>MYSTAVLLNKISPTRDGQTMTLADLQYLSFSELRKIFDDQLSWGEARHLYHETIEQKKNNRLLEARIFTRANPQLSGAIRLGIERDSVSRSYDEMFGARSSSFVKPGSVASMFSPAGYLTELYREAKDLHFSSSAYHLDNRRPDLADLTLSQSNMDTEISTLTLSNELLLEHITRKTGGDSDALMESLSTYRQAIDTPYHQPYETIRQVIMTHDSTLSALSRNPEVMGQAEGASLLAILANISPELYNILTEEITEKNADALFAQNFSENITPENFASQSWIAKYYGLELSEVQKYLGMLQNGYSDSTSAYVDNISTGLVVNNESKLEAYKITRVKTDDYDKNINYFDLMYEGNNQFFIRANFKVSREFGATLRKNAGPSGIVGSLSGPLIANTNFKSNYLSNISDSEYKNGVKIYAYRYTSSTSATNQGGGIFTFESYPLTIFALKLNKAIRLCLTSGLSPNELQTIVRSDNAQGIINDSVLTKVFYTLFYSHRYALSFDDAQVLNGSVINQYADDDSVSHFNRLFNTPPLKGKIFEADGNTVSIDPDEEQSTFARSALMRGLGVNSGELYQLGKLAGVLDAQNTITLSVFVISSLYRLTLLARVHQLTVNELCMLYGLSPFNGKTTASLSSGELPRLVIWLYQVTQWLTEAEITTEAIWLLCTPEFSGNISPEISNLLNNLRPSISEDMAQSHNRELQAEILAPFIAATLHLASPDMARYILLWTDNLRPGGLDIAGFMTLVLKESLNANETTQLVQFCHVMAQLSLSVQTLRLSEAELSVLVISGFAVLGAKNQPAGQHNIDTLFSLYRFHQWINGLGNPGSDTLDMLRQQTLTADRLASVMGLDISMVTQAMVSAGVNQLQCWQDINTVLQWIDVASALHTMPSVIRTLVNIRYVTALNKAESNLPSWDEWQTLAENMEAGLSTQQAQTLADYTAERLSSVLCNWFLANIQPEGVSLHSRDDLYSYFLIDNQVSSAIKTTRLAEAIAGIQLYINRALNRIEPNARADVSTRQFFTDWTVNNRYSTWGGVSRLVYYPENYIDPTQRIGQTRMMDELLENISQSKLSRDTVEDAFKTYLTRFETVADLKVVSAYHDNVNSNTGLTWFVGQTRENLPEYYWRNVDISRMQAGELAANAWKEWTKIDTAVNPYKDAIRPVIFRERLHLIWVEKEEVAKNGTDPVETYDRFTLKLAFLRHDGSWSAPWSYDITTQVEAVTDKKPDTERLALAASGFQGEDTLLVFVYKTGKSYSDFGGSNKNVAGMTIYGDGSFKKMENTALSRYSQLKNTFDIIHTQGNDLVRKASYRFAQDFEVPASLNMGSAIGDDSLTVMENGNIPQITSKYSSDNLAITLHNAAFTVRYDGSGNVIRNKQISAMKLTGVDGKSQYGNAFIIANTVKHYGGYSDLGGPITVYNKTKNYIASVQGHLMNADYTRRLILTPVENNYYARLFEFPFSPNTILNTVFTVGSNKTSDFKKCSYAVDGNNSQGFQIFSSYQSSGWLDIDTGINNTDIKITVMAGSKTHTFTASDHIASLPANSFDAMPYTFKPLEIDASSLAFTNNIAPLDIVFETKAKDGRVLGKIKQTLSVKRVNYNPEDILFLRETHSGAQYMQLGVYRIRLNTLLASQLVSRANTGIDTILTMETQRLPEPPLGEGFFANFVLPKYDPAEHGDERWFKIHIGNVGGNTGRQPYYSGMLSDTSETSMTLFVPYAEGYYMHEGVRLGVGYQKITYDNTWESAFFYFDETKQQFVLINDADHDSGMTQQGIVKNIKKYKGFLNVSIATGYSAPMDFNSASALYYWELFYYTPMMCFQRLLQEKQFDEATQWINYVYNPAGYIVNGEIAPWIWNCRPLEETTSWNANPLDAIDPDAVAQNDPMHYKIATFMRLLDQLILRGDMAYRELTRDALNEAKMWYVRTLELLGDEPEDYGSQQWAAPSLSGAASQTVQAAYQQDLTMLGRGGVSKNLRTANSLVGLFLPEYNPALTDYWQTLRLRLFNLRHNLSIDGQPLSLAIYAEPTDPKALLTSMVQASQGGSAVLPGTLSLYRFPVMLERTRNLVAQLTQFGTSLLSMAEHDDADELTTLLLQQGMELATQSIRI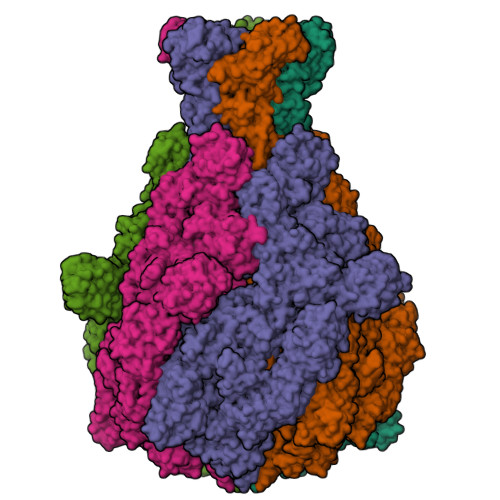QQRTVDEVDADIAVLAESRRSAQNRLEKYQQLYDEDINHGEQRAMSLLDAAAGQSLAGQVLSIAEGVADLVPNVFGLACGGSRWGAALRASASVMSLSATASQYSADKISRSEAYRRRRQEWEIQRDNADGEVKQMDAQLESLKIRREAAQMQVEYQETQQAHTQAQLELLQRKFTNKALYSWMRGKLSAIYYQFFDLTQSFCLMAQEALRRELTDNGVTFIRGGAWNGTTAGLMAGETLLLNLAEMEKVWLERDERALEVTRTVSLAQFYQALSSDNFNLTEKLTQFLREGKGNVGASGNELKLSNRQIEASVRLSDLKIFSDYPESLGNTRQLKQVSVTLPALVGPYEDIRAVLNYGGSIVMPRGCSAIALSHGVNDSGQFMLDFNDSRYLPFEGISVNDSGSLTLSFPDATDRQKALLESLSDIILHIRYTIRS[5x]> MESLTLQPIARVDGTINLPGSKSVSNRALLLAALAHGKTVLTNLLDSDDVRHMLNALTALGVSYTLSADRTRCEIIGNGGPLHAEGALELFLGNAGTAMRLLAAALCLGSNDIVLTGEPRMKERPIGHLVDALRLGGAKITYLEQENYPPLRLQGGFTGGNVDVDGSVSSQFLTALLMTAPLAPEDTVIRIKGDLVSKPYIDITLNLMKTFGVEIENQHYQQFVVKGGQSYQSPGTYLVEGDASSAS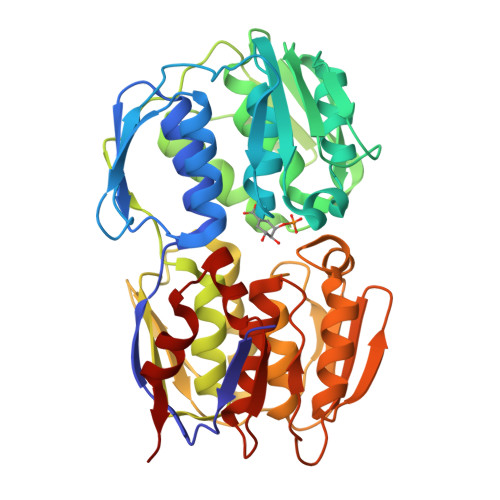YFLAAAAIKGGTVKVTGIGRNSMQGDIRFADVLEKMGATICWGDDYISCTRGELNAIDMDMNHIPDAAMTIATAALFAKGTTTLRNIYNWRVKETDRLFAMATELRKVGAEVEEGHDYIRITPPEKLNFAEIATYNDHRMAMCFSLVALSDTPVTILDPKCTAKTFPDYFEQLARISQAA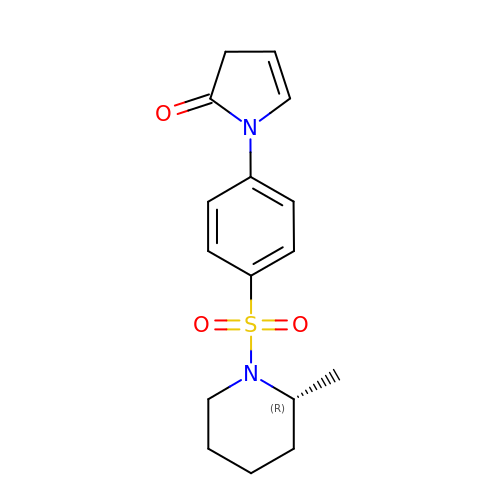1-(4-{[(2R)-2-methylpiperidin-1-yl]sulfonyl}phenyl)-1,3-dihydro-2H-pyrrol-2-one | C16 H20 N2 O3 S | MCVNUKURBWEELF-CYBMUJFWSA-N>[2x]TSTKRFTCPEESEASNCSCEEFPSKTHFYCPDFNPTLYVDVEDRMRVDFKCYDEPHDFKSLPNLAIGSVKLLTVVDCVLDDDRPILESFKFLEVADVRSFVYNNHENGIRYNAKYFEGMEQLENLTLARGVVSIDRDTFSGFLNLKRLTIEHNKLNLQPGTFEALSNLTYLGLVYNGLNEIQPGLFDGLESL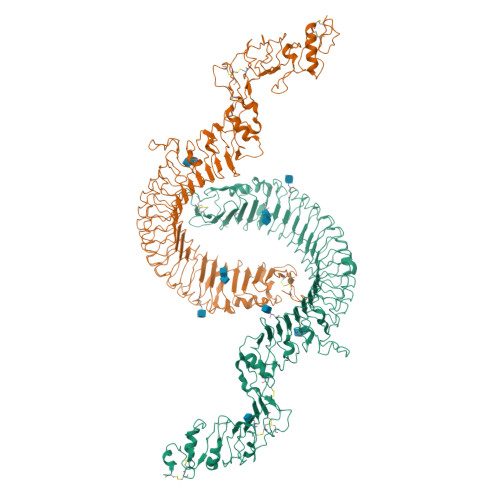EALSLSYNDIKSLSAGSFNGLSSLRMLNLRVNKIESFDANTFASLKELSRLEITLNPFVSLPRGLFSENKKLKTLILTNNRKLVTLPEELLANLKELTVVNLSHNGVGNLPESLLSGSSGIIELNLGYNRLNSLPEELLSDQPQLQVLNLDHNQLESIPDYFLERNVELQTLYLSHNRLRSLSEKAFTKLKNLKELHLENNQLQTIPQFLFSGTPKLEEIYMQNNQLALHANSFINEELSIADNDNTPFQVLQKLRILHLRNNSISTIFQDWYINNLEMQSLDLSFNKLPGLSYTQLQFQSNITLNLSNNEISQVLLIDDLDLQPYQRINVDLNHNPLNCNCNALKFIQLIQSKAEHGLQFNVDQLRCSEPPNLLDATMDQLQTKDLLCDFESADDCPKDCQCAMRLLDHTVIVNCSGRGLTEFPDLPIPSQLHEDFNALEVHVENNRLTKLPNLTKHNEITQLYARNNSIQNLLPHNIPSKLRIIDLSQNLLKMIDDSTLAQINRSSHLETIRLSQNQWLCDCPASSFLIFVQQNSRLISDMSAIRCHPSGKSLDSITVNELCFEDYTTENLYFQ> MNPPWAKPFELLVSFLNTPKYGTFDPTPVVPVFFPFWFGMIVGDIGYALLFYLVGRWLSGYVKRNEPLVIDLFALKLKPQVIGKLVHILNWMVFWTVVWGVIYGEFFGTFLEHLGVFGTPEHPGLIPILIHRIDTAKTANLLILLSVAFGVVLVFFGLALRAYLGLKHRHMAHFWEGVGYLGGLVGVLALAASYLGNLQAGWLQGLMYLGFGVFLLAVLMSRIWLMIPEIFTQAGHILSHIRIYAVGAAGGILAGLLTDVGFALAERLGLLGVLLGLLVAGVLHLLILLLTTLGHMLQPIRLL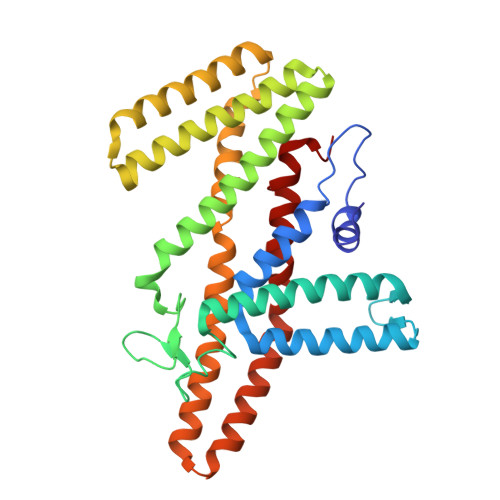WVEFFTKFGFYE>KLNDSNLFRQQALINGEWLDANNGEAIDVTNPANGDKLGSVPKMGADETRAAIDAANRALPAWRALTAKERATILRNWFNLMMEHQDDLARLMTLEQGKPLAEAKGEISYAASFIEWFAEEGKRIYGDTIPGHQADKRLIVIKQPIGVTAAITPWNFPAAMITRKAGPALAAGCTMVLKPASQTPFSALALAELAIRAGVPAGVFNVVTGSAGAVGNELTSNPLVRKLSFTGSTEIGRQLMEQCAKDIKKVSLELGGNAPFIVFDDADLDKAVEGALASKFRNAGQTCVCANRLYVQDGVYDRFAEKLQQAMSKLHIGDGLDNGVTIGPLIDEKAVAKVEEHIADALEKGARVVCGGKAHERGGNFF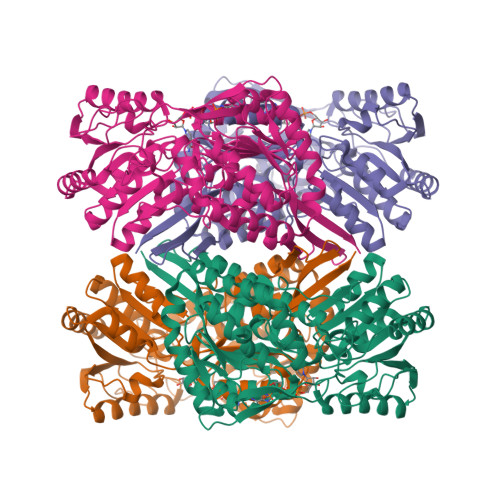QPTILVDVPANAKVSKEETFGPLAPLFRFKDEADVIAQANDTEFGLAAYFYARDLSRVFRVGEALEYGIVGINTGIISNEVAPFGGIKASGLGREGSKYGIEDYLEIKYMCIGL[4x]> AM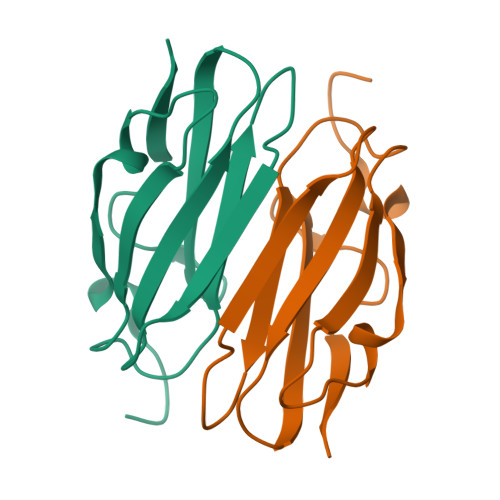GSDASKVVTRGPGLSQAFVGQKNSFTVDCSKAGTNMMMVGVHGPKTPCEEVYVKHMGNRVYNVTYTVKEKGDYILIVKWGDESVPGSPFKVKVP> AMGSRLYDRRSIFDAVAQSNCQELESLLPFLQRSKKRLTDSEFKDPETGKTCLLKAMLNLHNGQNDTIALLLDVARKTDSLKQFVNASYTDSYYKGQTALHIAIERRNMTLVTLLVENGADVQAAANGDFFKKTKGRPGFYFGELPLSLAACTNQLAIVKFLLQNSWQPADISARD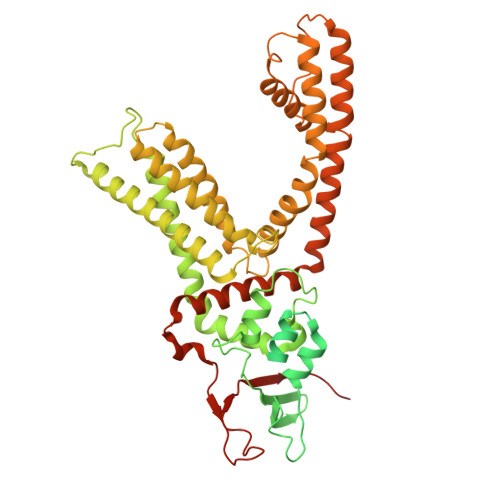SVGNTVLHALVEVADNTVDNTKFVTSMYNEILILGAKLHPTLKLEEITNRKGLTPLALAASSGKIGVLAYILQREIHEPECRHLSRKFTEWAYGPVHSSLYDLSCIDTCEKNSVLEVIAYSSSETPNRHDMLLVEPLNRLLQDKWDRFVKRIFYFNFFVYCLYMIIFTAAAYYRPVEGLPPYKLKNTVGDYFRVTGEILSVSGGVYFFFRGIQYFLQRRPSLKSLFVDSYSEILFFVQSLFMLVSVVLYFSQRKEYVASMVFSLAMGWTNMLYYTRGFQQMGIYAVMIEKMILRDLCRFMFVYLVFLFGFSTAVVTLIEDGKYNSLYSTCLELFKFTIGMGDLEFTENYDFKAVFIILLLAYVILTYILLLNMLIALMGETVNKIAQESKNIWKLQRAITILDTEKSFLKCMRKAFRSGKLLQVGFTPDGKDDYRWCFRVDEVNWTTWNTNVGIINEDPG>QIR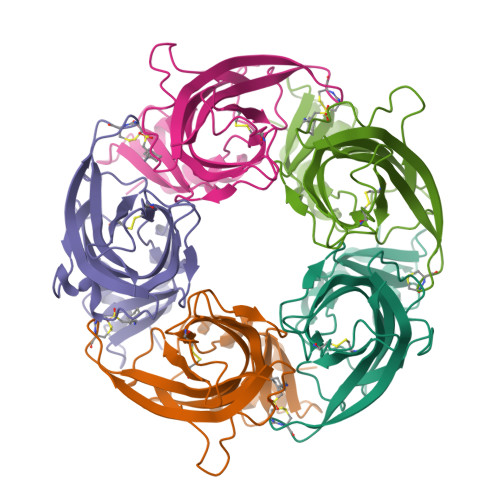WTLLNQITGESDVIPLSNNTPLNVSLNFKLMNIVEADTEKDQVEVVLWTQASWKVPYYSSLLSSSSLDQVSLPVSKMWTPDLSFYNAIAAPELLSADRVVVSKDGSVIYVPSQRVRFTCDLINVDTEPGATCRIKVGSWTHDNKQFALITGEEGVVNIAEYFDSPKFDLLSATQSLNRKKYSCCENMYDDIEITFAFRKK[5x]5-(2-chlorophenyl)-N-hydroxy-1,3-oxazole-2-carboxamide | C10 H7 Cl N2 O3 | 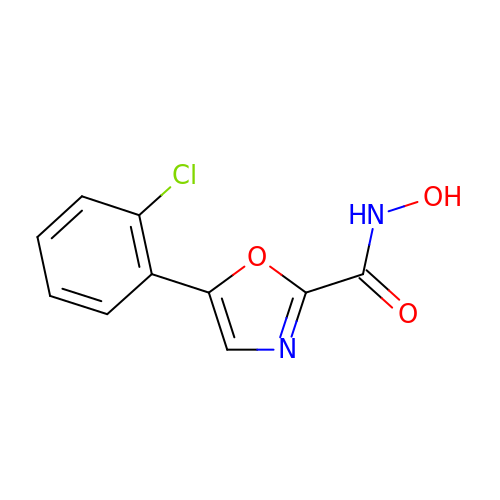OZEMICSCADZYKS-UHFFFAOYSA-N> MGVSPAAPASGIRRPCYLVLSSHDFRTPRRANIHFITDQLALRGTTRFFSLRYSRLSRMKGDMRLPLDDTANTVVSHNGVDCYL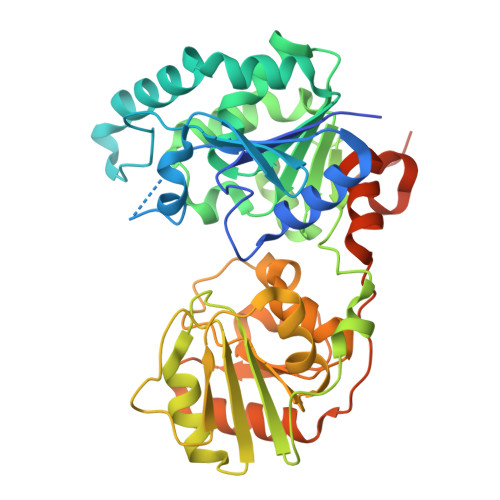WRTTVHPFNTRRSWLRPVEDAMFRWYAAHPPKQLLDWMRESDVIVFESGIAVAFIELAKRVNPAAKLVYRASAGLSTINVASYIEREFDRVAPTLDVIALVSPAMAAEVVSRDNVFHVGHGVDHNLDQLGDPSPYAEGIHAVAVGSMLFDPEFFVVASKAFPQVTFHVIGSGMGRHPGYGDNVIVYGEMKHAQTIGYIKHARFGIAPYASEQVPVYLADSSMKLLQYDFFGLPAVCPNAVVGPYKSRFGYTPGNADSVIAAITQALEAPRVRYRQCLNWSDTTDRVLDPRAYPETRLYPHPPTAAPQLSSEAALSHHHHHHH> LKIAAFNIRTFGETKMSNATLASYIVRIVRRYDIVLIQEVRDSHLVAVGKLLDYLNQDDPNTYHYVVSEPLGRNSYKERYLFLFRPNKVSVLDTYQYDDGCESCGNDSFSREPAVVKFSSHSTKVKEFAIVALHSAPSDAVAEINSLYDVYLDVQQKWHLNDVMLMGDFNADCSYVTSSQWSSIRLRTSSTF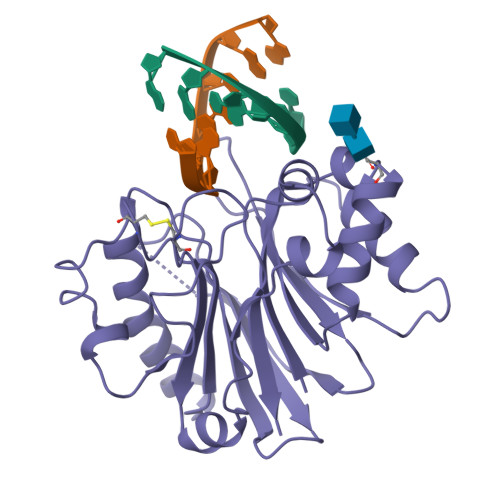QWLIPDSADTTATSTNCAYDRIVVAGSLLQSSVVPGSAAPFDFQAAYGLSNEMALAISDHYPVEVTLT>HMPRVLVTGALGQIGTDLSLALRDKFGADSVLVSDVVEPGAKHPLAGLKGVEKLDCLDSNGFEKLVKEFKPTWMYHLPAIMSVRGEAEPDLAMDINVNTTRYALELARKYNIRIFIPSTIAAFGDKCGKTMTKDDTIMNPSTVYGVTKVYTELLGTWYRQKYGVDFRSVRLPGIISAA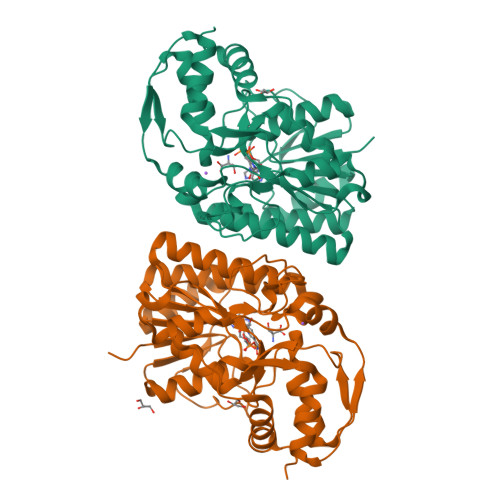TLPGGGATDYAIHMYHSALLQKKCVCPVLPYESLPMMYMPDTLNSLVKIMEAPLEKLTRTVYNITGFSFSPSELRFSIERCTDRTIEVEYVEGPAQKIANSWPDSLDDSNARNDWGHQVKYDIDMMSEDMLRQIPILHGLPSL[2x]> MDLQLKQAKLRLLYFNIRGRAELIRLVLNAAEKDFEDVRVSETEWPSLKSKMPFNQLPVLEVTTPNGQKVMLTESMAIARLLARTFGLYGDNAAEVYLIERMNSLTSSLLEEIYALGLKKVDSFKKLFE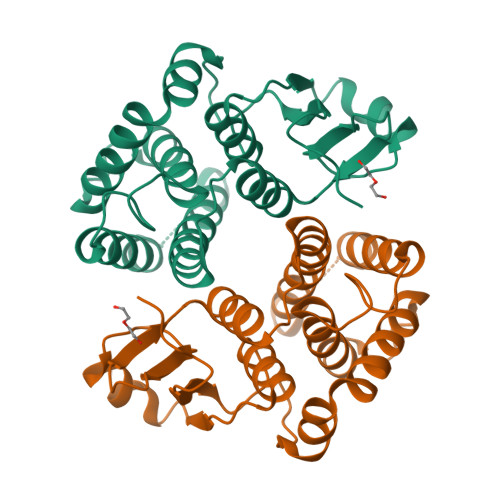AEHLHEYMNAIEMALKERKSTFIAGPRVTLADLQVIVLIDTMNKFLPNTKHECKDKLDEIKEGVIRTKPGVARYLRSRPATDF>[2x]UGGGGU

G-quadruplexes (G4s) are a class of four-stranded secondary structures that can form within guanine-rich nucleic acids. DHX36 is a member of the DEAH-box helicase family and exhibits adenosine triphosphate (ATP)-dependent, G4-specific unwinding activity in vitro. In vitro characterization of DHX36 revealed that the helicase binds G4 substrates with remarkably low, picomolar dissociation constants and only unwinds DNA and RNA G4s. Furthermore, we find that ATP consumption by DHX36 is largely independent of G4 stability. Together, we propose that DHX36 unwinds G4 nucleic acids using a mechanism similar to that employed by homologous DEAD-box helicases that act on double-stranded nucleic acids.

Tetramolecular G4 substrates were chosen for their kinetic stability and straightforward characterization through native PAGE. Tetramolecular G4s are commonly used for the study of protein or small molecule recognition of G4s. All tetramolecular G4 substrates were shown to adopt a parallel G4 topology by circular dichroism (CD) spectroscopy. The core of the G4s is composed of stacked guanine tetrads as exemplified by the crystal structure of r[UGGGGU]4 presented in Figure 1B. The X-ray structure of r[UGGGGU]4, now determined at 1.08 Å resolution using crystals grown in the presence of the physiological cation, K+, confirms that it adopts a parallel, all anti-glycosidic conformation. (A structure of the same oligonucleotide forming a quadruplex bound to Sr2+ has been reported previously). Since the formation of G4 structures is enthalpically driven, with a per-tetrad ΔΔH of -20 to -25 kcal·mol−1 (30), increasing the number of guanine tetrads thus increases the thermodynamic stability of the formed G4.> QPIFLNVLEAIEPGVVCAGHDNNQPDSFAALLSSLNELGERQLVHVVKWAKALPGFRNLHVDDQMAVIQYSWMGLMVFAMGWRSFTNVNSAMLYFAPDLVFNEYRMHKSRMY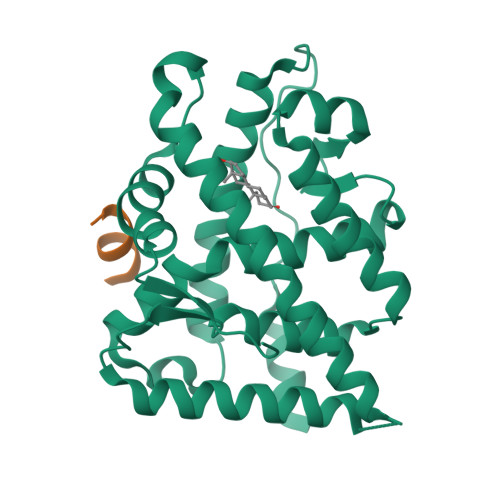SQCVRMRHLSQEFGWLQITPQEFLCMKALLLFSIIPVDGLKNQKFFDELRMNYIKELDRIIACKRKNPTSCSRRFYQLTKLLDSVQPIARELHQFTFDLLIKSHMVSVDFPEMMAEIISVQVPKILSGKVKPIYFHTQ;> SDSAFSRYYTRS The bacteriophage T7, Escherichia coli podophage, has been employed as a model for the investigation of the DNA packaging and delivery mechanism among tailed phages and related dsDNA viruses. The tail, connected to a unique vertex of the head by the dodecameric portal gp8, consists of the dodecameric adaptor protein gp11 and the hexameric nozzle protein gp12 (20, 24) surrounded by six trimeric tail fibers gp17 (16, 22, 24). The core is formed by the core proteins gp14, gp15, and gp16; upon virion adsorption onto host membranes or the receptor rough lipopolysaccharide (LPS), these core proteins have been suggested to extend the tail channel and form a trans-envelope channel for genome delivery into the infected cell. In this study, using a 300 kV cryo-electron microscopy (cryo-EM) and defocus refinement with Z-height correction, we provided improved structures of core proteins at a resolution of 3 Å, the portal–tail complex in mature T7 at a resolution of 2.7 Å, and the portal–tail complex in LPS-induced DNA-ejected T7 at a resolution of 3.5 Å.

The core in mature T7 is formed by a four-fold gp16 ring, an eight-fold gp15 ring, and a less-well-defined eight-fold spoke, which could be formed by gp14 (23). On the basis of our improved density map, we identified eight copies of gp14 between the gp15 ring and the portal helical barrel. We also modeled 112 amino acid residues (4–86 and 101–129) of the 196-residue gp14 protein. Each gp14 molecule is composed of five α-helices connected by four loops. The longest helix α1 and a shorter helix α2 in the gp14 molecule enwind the portal barrel, bridging the portal barrel and the sidewall of the cylinder formed by gp15. Helix α3 traverses through a hole on the sidewall, and helices α4 and α5 bind to the outer sidewall of the cylinder, which is surrounded by the genomic DNA. Intriguingly, only eight copies of the gp6.7 loop II were resolved to interact with the inner sidewall of the cylinder formed by gp15. Thus, gp6.7 serves as an adapter for coordinating the symmetry mismatch between the dodecameric helical barrel domain of the portal, the eight copies of gp14, and the eight copies of gp15, thereby stabilizing the core proteins on the portal. We speculate that the eight copies of gp14 are to adapt the symmetry–mismatch between the twelve-fold ring of gp6.7 loop I around the portal and eightfold ring of gp15 during the core assembly.

>[8x]MCFSPKIKTPKMDTNQIRAVEPAPLTQEVSSVEFGGSSDETDTEGTEVSGRKGLKVERDDSVAKSKASGNGSARMKSSIRKSAFGGKK;>[8x]MSKIESALQAAQPGLSRLRGGAGGMGYRAATTQAEQPRSSLLDTIGRFAKAGADMYTAKEQRARDLADERSNEIIRKLTPEQRREALNNGTLLYQDDPYAMEALRVKTGRNAAYLVDDDVMQKIKEGVFRTREEMEEYRHSRLQEGAKVYAEQFGIDPEDVDYQRGFNGDITERNISLYGAHDNFLSQQAQKGAIMNSRVELNGVLQDPDMLRRPDSADFFEKYIDNGLVTGAIPSDAQATQLISQAFSDASSRAGGADFLMRVGDKKVTLNGATTTYRELIGEEQWNALMVTAQRSQFETDAKLNEQYRLKINSALNQEDPRTAWEMLQGIKAELDKVQPDEQMTPQREWLISAQEQVQNQMNAWTKAQAKALDDSMKSMNKLDVIDKQFQKRINGEWVSTDFKDMPVNENTGEFKHSDMVNYANKKLAEIDSMDIPDGAKDAMKLKYLQADSKDGAFRTAIGTMVTDAGQEWSAAVINGKLPERTPAMDALRRIRNADPQLIAALYPDQAELFLTMDMMDKQGIDPQVILDADRLTVKRSKEQRFEDDKAFESALNASKAPEIARMPASLRESARKIYDSVKYRSGNESMAMEQMTKFLKESTYTFTGDDVDGDTVGVIPKNMMQVNSDPKSWEQGRDILEEARKGIIASNPWITNKQLTMYSQGDSIYLMDTTGQVRVRYDKELLSKVWSENQKKLEEKAREKALADVNKRAPIVAATKAREAAAKRVREKRKQTPKFIYGRKE;>[4x]MDKYDKNVPSDYDGLFQKAADANGVSYDLLRKVAWTESRFVPTAKSKTGPLGMMQFTKATAKALGLRVTDGPDDDRLNPELAINAAAKQLAGLVGKFDGDELKAALAYNQGEGRLGNPQLEAYSKGDFASISEEGRNYMRNLLDVAKSPMAGQLETFGGITPKGKGIPAEVGLAGIGHKQKVTQELPESTSFDVKGIEQEATAKPFAKDFWETHGETLDEYNSRSTFFGFKNAAEAELSNSVAGMAFRAGRLDNGFDVFKDTITPTRWNSHIWTPEELEKIRTEVKNPAYINVVTGGSPENLDDLIKLANENFENDSRAAEAGLGAKLSAGIIGAGVDPLSYVPMVGVTGKGFKLINKALVVGAESAALNVASEGLRTSVAGGDADYAGAALGGFVFGAGMSAISDAVAAGLKRSKPEAEFDNEFIGPMMRLEARETARNANSADLSRMNTENMKFEGEHNGVPYEDLPTERGAVVLHDGSVLSASNPINPKTLKEFSEVDPEKAARGIKLAGFTEIGLKTLGSDDADIRRVAIDLVRSPTGMQSGASGKFGATASDIHERLHGTDQRTYNDLYKAMSDAMKDPEFSTGGAKMSREETRYTIYRRAALAIERPELQKALTPSERIVMDIIKRHFDTKRELMENPAIFGNTKAVSIFPESRHKGTYVPHVYDRHAKALMIQRYGAEGLQEGIARSWMNSYVSRPEVKARVDEMLKELHGVKEVTPEMVEKYAMDKAYGISHSDQFTNSSIIEENIEGLVGIENNSFLEARNLFDSDLSITMPDGQQFSVNDLRDFDMFRIMPAYDRRVNGDIAIMGSTGKTTKELKDEILALKAKAEGDGKKTGEVHALMDTVKILTGRARRNQDTVWETSLRAINDLGFFAKNAYMGAQNITEIAGMIVTGNVRALGHGIPILRDTLYKSKPVSAKELKELHASLFGKEVDQLIRPKRADIVQRLREATDTGPAVANIVGTLKYSTQELAARSPWTKLLNGTTNYLLDAARQGMLGDVISATLTGKTTRWEKEGFLRGASVTPEQMAGIKSLIKEHMVRGEDGKFTVKDKQAFSMDPRAMDLWRLADKVADEAMLRPHKVSLQDSHAFGALGKMVMQFKSFTIKSLNSKFLRTFYDGYKNNRAIDAALSIITSMGLAGGFYAMAAHVKAYALPKEKRKEYLERALDPTMIAHAALSRSSQLGAPLAMVDLVGGVLGFESSKMARSTILPKDTVKERDPNKPYTSREVMGAMGSNLLEQMPSAGFVANVGATLMNAAGVVNSPNKATEQDFMTGLMNSTKELVPNDPLTQQLVLKIYEANGVNLRERRK;>[8x]MCWAAAIPIAISGAQAISGQNAQAKMIAAQTAAGRRQAMEIMRQTNIQNADLSLQARSKLEEASAELTSQNMQKVQAIGSIRAAIGESMLEGSSMDRIKRVTEGQFIREANMVTENYRRDYQAIFAQQLGGTQSAASQIDEIYKSEQKQKSKLQMVLDPLAIMGSSAASAYASGAFDSKSTTKAPIVAAKGTKTGR During glycolysis, pyruvate kinase (PK) catalyzes the irreversible phosphorylation of ADP at the expense of phosphoenolpyruvate (PEP), yielding pyruvate and ATP. Previous characterization of cytoplasmic T. gondii pyruvate kinase (TgPK1), using either parasite extracts or a recombinant purified enzyme, indicated that this enzyme was allosterically activated by glucose 6-phosphate (G6P), which enhanced its activity under PEP unsaturated conditions. We solved the structure of two different constructs of TgPK1: the full-length enzyme (Met1 to Glu531 plus its N-terminal 6×His tag), which crystallized in the absence of substrates, effectors or added ions (“full TgPK1”); and an N-terminal truncated version starting at position Ile39 (“truncated TgPK1”). In both crystals, the asymmetric unit is composed of a tetramer with imperfect D2 symmetry.

Crystals of the truncated TgPK1 were grown in the presence of K+, Mg2+ and a potential inhibitor, although no evidence for this compound was found in the electron density. Conversely, in the truncated TgPK1 structure all of the B domains were visible in the electron density, with one monomer remarkably displaying a closed conformation for this domain. This large structural rearrangement involving a rigid body motion of the B domain resulted in a maximum displacement of nearly 20 Å (Fig. 3 and supplementary Datapack S1). Steric hindrance effects would prevent the binding of the nucleotide to this conformation; consequently we defined it as inactive. Two hinge bending motion regions were identified containing two conserved Pro residues, P125 and P216, at which point the B domain pivots towards the A domain by rotating ∼68°, generating a 77% closed conformation compared to the open conformation. Finally, a disordered region was exclusively associated with the closing of the AB cleft in the truncated TgPK1, the Gly300 to Ile306 loop. In the disordered conformation, additional electron density was observed and modeled as a sulfate molecule binding three side chain hydroxyl groups of residues Thr437, Thr439 and Thr442. In the new conformation present in the truncated TgPK1, when the Lys515-Ser522 is ordered, the carboxylate group of Glu516 occupies the position of the sulfate group.

>[4x]MHHHHHHSSGRENLYFQGIRMSQILEPRSEEDWTAHRTRIVCTMGPACWNVDTLVKMIDAGMNVCRLNFSHGDHETHARTVQNIQEAMKQRPEARLAILLDTKGPEIRTGFLKDHKPITLQQGATLKIVTDYNLIGDETTIACSYGALPQSVKPGNTILIADGSLSVKVVEVGSDYVITQAQNTATIGERKNMNLPNVKVQLPVIGEKDKHDILNFGIPMGCNFIAASFVQSADDVRYIRGLLGPRGRHIRIIPKIENVEGLVNFDEILAEADGIMIARGDLGMEIPPEKVFLAQKMMIAKCNVVGKPVITATQMLESMIKNPRPTRAEAADVANAVLDGTDCVMLSGETANGEFPVITVETMARICYEAETCVDYPALYRAMCLAVPPPISTQEAVARAAVETAECVNAAIILALTETGQTARLIAKYRPMQPILALSASESTIKHLQVIRGVTTMQVPSFQGTDHVIRNAIVVAKERELVTEGESIVAVHGMKEEVAGSSNLLKVLTVE>TEKKYIVALDQGTTSSRAVVMDHDANIISVSQREFEQIYPKPGWVEHDPMEIWATQSSTLVEVLAKADISSDQIAAIGITNQRETTIVWEKETGKPIYNAIVWQCRRTAEICEHLKRDGLEDYIRSNTGLVIDPYFSGTKVKWILDHVEGSRERARRGELLFGTVDTWLIWKMTQGRVHVTDYTNASRTMLFNIHTLDWDDKMLEVLDIPREMLPEVRRSSEVYGQTNIGGKGGTRIPISGIAGDQQAALFGQLCVKEGMAKNT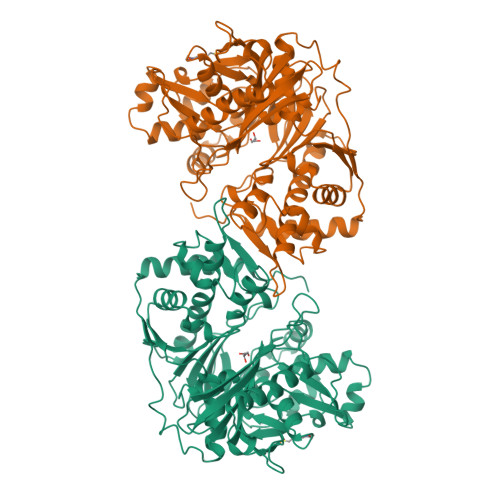YGTGCFMLMNTGEKAVKSENGLLTTIACGPTGEVNYALEGAVFMAGASIQWLRDEMKLINDAYDSEYFATKVQNTNGVYVVPAFTGLGAPYWDPYARGAIFGLTRGVNANHIIRATLESIAYQTRDVLEAMQADSGIRLHALRVDGGAVANNFLMQFQSDILGTRVERPEVREVTALGAAYLAGLAVGFWQNLDELQEKAVIEREFRPGIETTERNYRYAGWKKAVKRAMAWEEHDE[2x]>GSHMASGDATDITIYYKTGWTHPHIHYSLNQGAWTTLPGVPLTKSEYEGYVKVTIEAEEGSQLRAAFNNGSGQWDNNQGRDYDFSS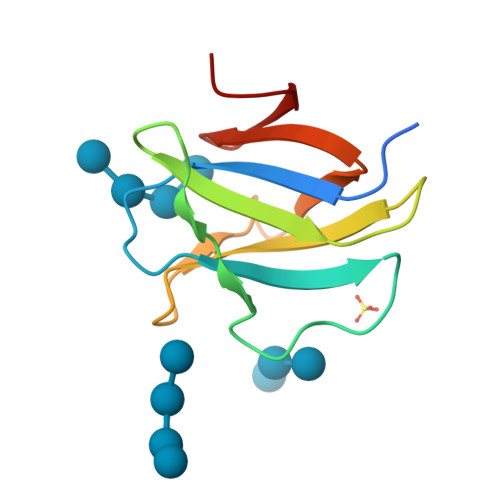GVHTLADGRILSGTPK[4x]> GTDLITLEMVFAANLNQDKSSCEAILPFLNEYAKTYGMKEERAMAHFLSQVGHESNFKPVSENLRYSPKGMRKIFGCKGGSKNYDPILDDAKEGRLRPKLWTHESDYAFNPVALGNYVYANRPGSKNGDESSGDGYKYRGRGLIQITHKDAYIKFTEAHNAANPSDQKDFLASPDDILTLRYATSSAYFFWFIYKKSFNLHSTACTGTVKEVTKIVNGGYAGYADRLKRFNAVAAVIGIDGARE

Here, we report that a T6SS effector TseP, from Aeromonas dhakensis, represents a family of effectors with dual amidase-lysozyme activities. Our previous findings have established that TseP serves a structural role because its expression can restore the T6SS secretion in the Δ3eff mutant lacking all three effector genes, and the C-terminal domain, TsePC, possesses lysozyme activities. However, the function of the N-terminal domain, TsePN, which lacks any recognizable conserved motif, has remained elusive. This study unveils that TsePN is capable of cleaving the peptide link between NAM and L-Ala as an amidase. TsePN, the N-terminal domain, functions as a Zn2+-dependent amidase, while the C-terminal domain, TsePC, exhibits lysozyme activities.

While testing TseP-mediated hydrolysis of purified PG from Gram-negative bacteria, we noticed that both TseP and TsePC displayed more efficient digestion than the commonly used hen-egg lysozyme. To further investigate this, we determined the X-ray crystal structure of TsePC to a resolution of 2.27 Å (Rwork = 0.189 and Rfree = 0.227) by molecular replacement with one molecule in the asymmetric unit. The crystal structure revealed that TsePC comprises a smaller lobe of seven helices and a larger lobe of ten helices, separated by a concave groove. The surface electrostatic potential of TsePC, calculated using the Adaptive Poisson-Boltzmann Solver (APBS), consists of both electronegative and electropositive regions, unlike the predominantly electronegative groove of lysozyme. The electropositive surface of TsePC consists of residues R723 and K796, with an adjacent residue Y720 corresponding to W62 in lysozyme, altering which is known to affect substrate binding. Additionally, the previously predicted catalytic dyad (E655 and E663) was located near the groove. Although this structural arrangement resembles that of other lysozyme family members, TsePC exhibits a less compact conformation with a notably wider groove compared to the typical lysozyme. Previous studies have shown that the lysozyme possesses catalytic sites at E53 and D70 in the substrate-binding groove, while the active residues in the TsePC structure are E654 and E663, respectively. To test the effect of E663 for TsePC activity, we purified a mutant E663D (TsePC-E663D) protein and perform PG-digestion assays. The results show that TsePC-E663D lost the activity, suggesting the greater distance within the groove requires this glutamate residue.>MERTFVMIKPDGVRRGLVGEILARFERKGFRIAALKLMQISQELAERHYAEHREKPFFPGLVRFITSGPVVAMVLEGPGVVAEVRKMMGATHPKDALPGTIRGDFATTIDENVIHGSATLEDAQREIALFF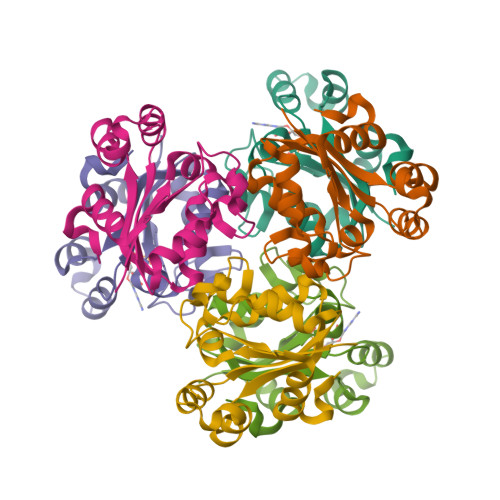RPEELL[2x]> GSMESAQAVAEPLDLVRLSLDEIVYVKLR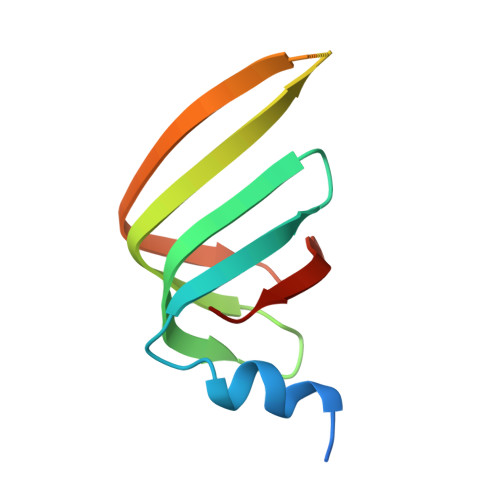GDRELNGRLHAYDEHLNMVLGDAEEIVTIFDDEETDKDKALKTIRKHYEMLFVRGDSVILIAPPRN> MKKLLVTVLLAVFGALAFAAEEAAASGGLDRGLIAVGMGLAVGLAALGTGV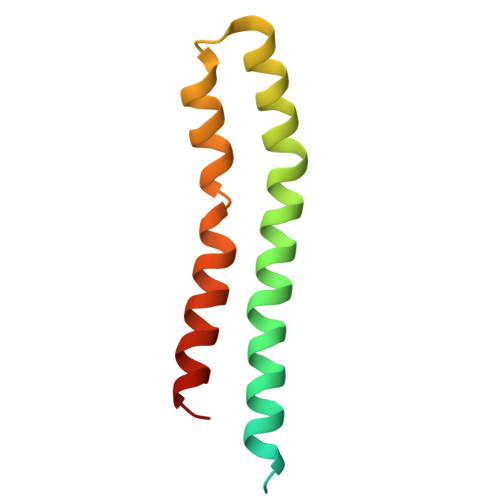AQARIGAAGVGAIAEDRSNFGTALIFLLLPETLVIFGLLIAFILNGRLHHH1-[(2S)-2-{[(2Z)-2-(2-amino-1,3-thiazol-4-yl)-2-{[(2-carboxypropan-2-yl)oxy]imino}acetyl]amino}-3-oxopropyl]-4-{[2-(5,6-dihydroxy-1,3-dioxo-1,3-dihydro-2H-isoindol-2-yl)ethyl]carbamoyl}-2,5-dihydro-1H-pyrazole-3-carboxylic acid | C27 H28 N8 O12 S | 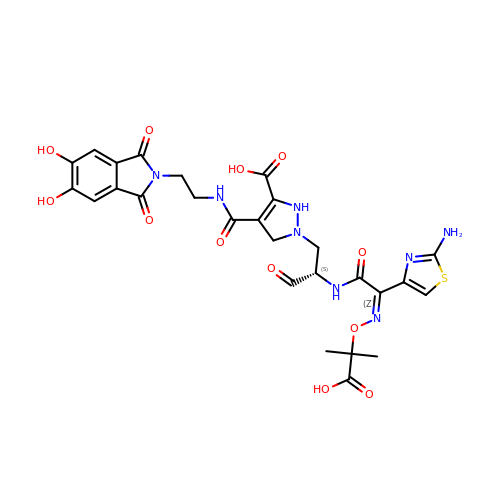AUDGPVZSFLGMAE-ZJIUGIBFSA-N>MDLLTAKTIVLGC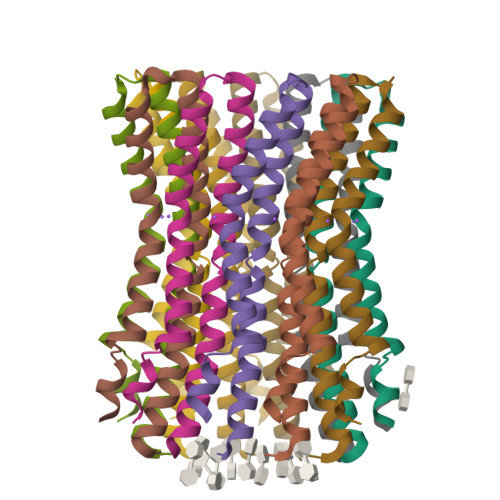SAVGAGLAMIAGLGPGIGEGYAAGKAVESVARQPEARGSIISTMILGQAVAESTGIYSLVIALILLYANPFLSKLG[22x]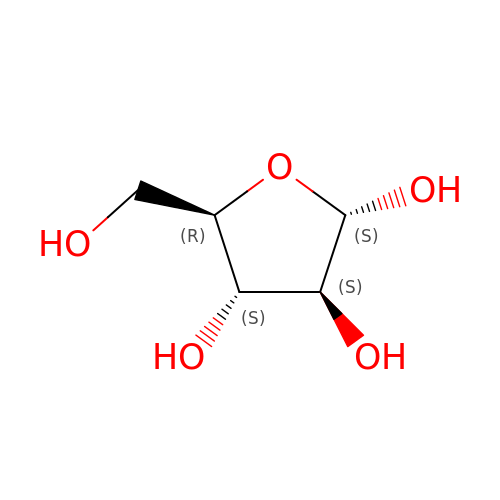alpha-D-arabinofuranose | C5 H10 O5 | HMFHBZSHGGEWLO-MBMOQRBOSA-N2-[3,4-bis(oxidanyl)phenyl]-3-[(2S,3R,4S,5R,6R)-6-(hydroxymethyl)-3,4,5-tris(oxidanyl)oxan-2-yl]oxy-5,7-bis(oxidanyl)chromen-4-one | C21 H20 O12 | 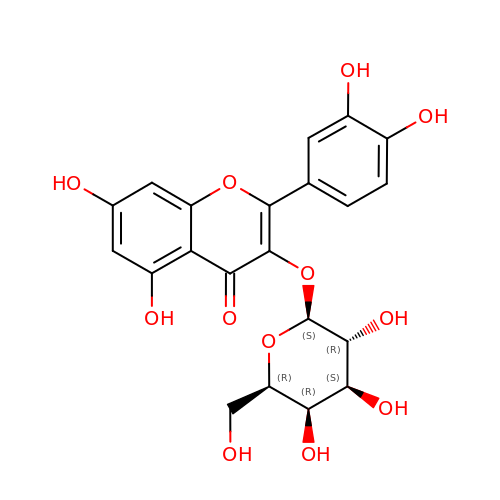OVSQVDMCBVZWGM-DTGCRPNFSA-N>MKALRGMISEKGGWNLTVNNDNNTVVSSGGALDLSSGSKNLKIVKDGKKNNVTFDVARDLTLKSIKLDGVTLNETGLFIANGPQITASGINAGSQKITGVAEGTDANDAVNFGQLKKIETEVKEQVAASGFVKQDSDTKYLTIGKDTDGDTINIANNKSDKRT[3x]

In Proteobacteria, colonization of the host depends on a wide range of adhesive surface molecules, among which Trimeric Autotransporter Adhesins (TAAs) represent a major class. All TAAs follow a head-stalk-anchor architecture in the direction from amino- to carboxy-terminus of the protein. The head, which is projected above the cell surface by the stalk, mediates a range of molecular interactions such as autoagglutination and attachment to host tissue, typically via proteins of the extracellular matrix, e.g. collagen, fibronectin, or laminin. Of the experimentally studied TAAs, Bartonella henselae BadA is the longest representative, at over 3000 residues, and extends approx. 240 nm from the bacterial cell surface.

We have determined the structure of two domains from the head of the Bartonella henselae adhesin BadA. To this end, we built full-atom models for each domain, as described in the Methods section. Molecular replacement searches returned two solutions, which were further refined, and a trimeric model of residues 385 to 498 of BadA could be built into the electron density map (underlined in Figure 2A). The termini of the construct were not resolved, as expected from the results of proteolytic digestion, which suggested that they are unstructured. The overall structure of the construct is rod-like, with a length of 10 nm and an approximate diameter of 2.5 nm. The three chains are tightly intertwined and each can only assume its structure in the context of the other two. The structure consists of four distinct elements, as anticipated from the sequence analysis: the Trp-ring domain, named for the peculiar arrangement of the highly conserved Trp residues, the GIN domain, a neck sequence, and a short segment of the coiled-coil stalk of BadA. The Trp-ring domain forms a β-prism of interleaved, five-stranded β-meanders parallel to the trimer axis. The GIN domain (residues 435–466) also forms a β-prism of 5-stranded β-meanders, albeit not interleaved and perpendicular to the trimer axis. The neck sequence serves as a connector, which makes the transition from the wide diameter of the β-prisms to the narrower diameter of the coiled-coil stalk. In our construct, we had included 50 residues from the N-terminal part of the BadA stalk, but only two heptads are visible in the structure, the rest being disordered.> MVAKGRIIRVTGPLVVADGMKGAKMYEVVRVGELGLIGEIIRLEGDKAVIQVYEETAGVRPGEPVVGTGASLSVELGPRLLTSIYDGIQRPLEVIREKTGDFIARGVTAPALPRDKKWHFIPKAKVGDKVVGGDIIGEVPETSIIVHKIMVPP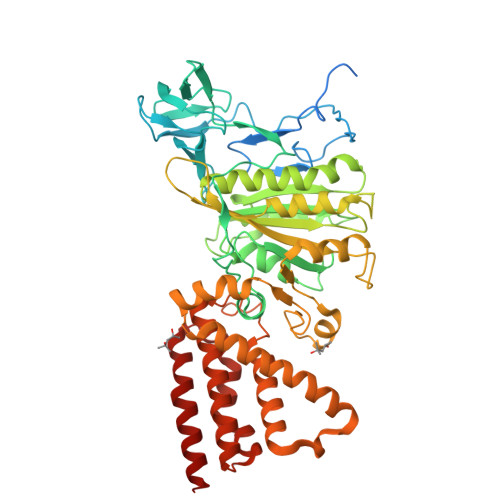GIEGEIVEIAEEGDYTIEEVIAKVKTPSGEIKELKMYQRWPVRVKRPYKEKLPPEVPLITGQRVIDTFFPQAKGGTAAIPGPFGSGKAVTQHQLAKWSDAQVVIYIGCGERGNEMTDVLEEFPKLKDPKTGKPLMERTVLIANTSNMPVAAREASIYTGITIAEYFRDMGYDVALMADSTSRWAEALREISGRLEEMPGEEGYPAYLASKLAEFYERAGRVVTLGSDYRVGSVSVIGAVSPPGGDFSEPVVQNTLRVVKVFWALDADLARRRHFPAINWLTSYSLYVDAVKDWWHKNIDPEWKAMRDKAMALLQKESELQEIVRIVGPDALPERERAILLVARMLREDYLQQDAFDEVDTYCPPEKQVTMMRVLLNFYDKTMEAINRGVPLEEIAKLPVREEIGRMKFERDVSKIRSLIDKTNEQFEELFKKYGA> EYDLKRLRNIGIAAHIDAGKTTTTERILYYTGRIAVTTCFWKDHRINIIDTPGHVDFTIEVERSMRVLDGAIVVFDSSQGVEPQSETVWRQAEKYKVPRIAFANKMDKTGADLWLVIRTMQERLGARPVVMQLPIGREDTFSGIIDVLRMKAYTYGNDLGTDIREIPIPEEYLDQAREYHEKLVEVAADFDENIMLKYLEGEEPTEEELVAAIRKGTIDLKITPVFLGSALKNKGVQLLLDAVVDYLPSPLDIPPIKGTTPEGEVVEIHPDPNGPLAALAFKIMADPYVGRLTFIRVYSGTLTSGSYVYNTTKGRKERVARLLRMH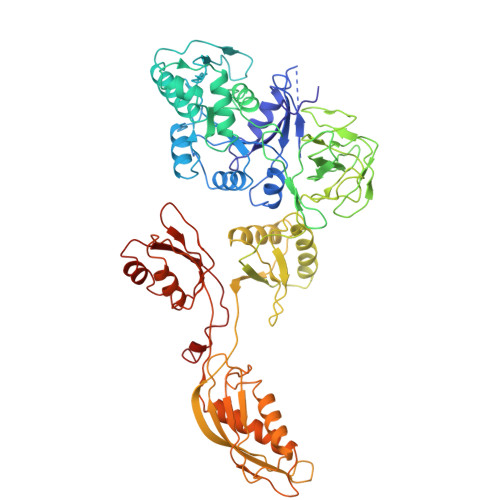ANHREEVEELKAGDLGAVVGLKETITGDTLVGEDAPRVILESIEVPEPVIDVAIEPKTKADQEKLSQALARLAEEDPTFRVSTHPETGQTIISGMGELHLEIIVDRLKREFKVDANVGKPQVAYRETITKPVDVEGKFIRQTGGRGQYGHVKIKVEPLPRGSGFEFVNAIVGGVIPKEYIPAVQKGIEEAMQSGPLIGFPVVDIKVTLYDGSYAEVDSSEMAFKIAGSMAIKEAVQKGDPVILEPIMRVEVTTPEEYMGDVIGDLNARRGQILGMEPRGNAQVIRAFVPLAEMFGYATDLRSKTQGRGSFVMFFDHYQEVPKQVQEKLI(1~{S},3~{S},4~{R},5~{R})-3-methyl-1,4,5-tris(hydroxyl)cyclohexane-1-carboxylic acid | C8 H14 O5 | 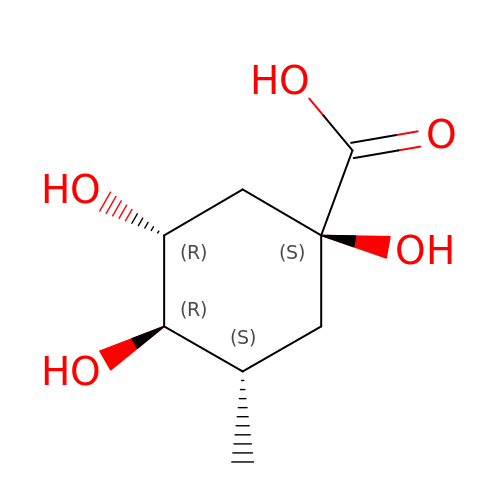NMVUNDOHFYILSF-FJDLHZNMSA-N>[2x]GPGPEYQAQGLAMYLQENGIDCPKCKFSYALARGGCMHFHCT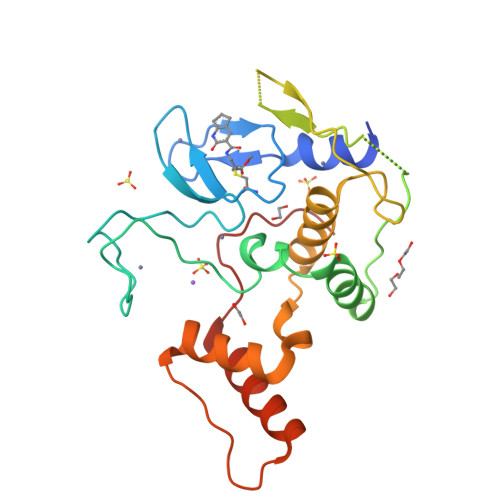QCRHQFCSGCYNAFYAKNKCPEPNCRVKKSLHGHHPRDCLFYLRDWTALRLQKLLQDNNVMFNTEPPAGARAVPGGGCRVIEQKEVPNGLRDEACGKETPAGYAGLCQAHYKEYLVSLINAHSLDPATLYEVEELETATERYLHVRPQPLAGEDPPAYQARLLQKLTEEVPLGQSIPRRRK>[2x]MSVLQVLTFPDDRLRTVAKPVEQVTPEI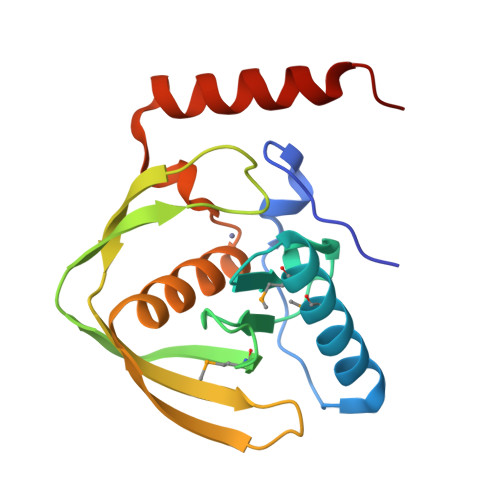QQIVDDMLETMYAEEGIGLAATQVDIHQRIVVIDISETRDQPMVLINPEIIEKRGEDGIEEGCLSVPGARALVPRAAEVTVKALDRNGQEYQFDADDLLAICVQHELDHLAGKLFVDYLSPLKRNRIKEKLEKIKRFNEKK Collagenase from the gram-negative bacterium Grimontia hollisae strain 1706B (Ghcol) degrades collagen more efficiently even than clostridial collagenase, the most widely used industrial collagenase. Collagenase (Enzyme Commission number: 3.4.24.3) cleaves the triple-helical region of collagen under physiological conditions, catalyzing the hydrolysis of peptide bonds with glycine residues at the P1 position. It produces the collagenase Ghcol, which consists of 767 amino acid residues with a single catalytic domain containing the zinc-binding motif H492EYVH496. Here, we report the crystal structures of ligand-free and Gly-Pro-hydroxyproline (Hyp)-complexed Ghcol at 2.2 and 2.4 Å resolution, respectively. These structures revealed that the activator and peptidase domains in Ghcol form a saddle-shaped structure with one zinc ion and four calcium ions.

Crystals of Ghcol complexed with Gly-Pro-Hyp were prepared by soaking the crystals of ligand-free Ghcol in a reservoir solution containing Gly-Pro-Hyp. Unexpectedly, Ghcol binds to two peptides at each of three binding sites, which are present in the active site (a) and in the activator subdomains, Act1 (b) and Act2 (c). The sites are separated by a distance of 15 to 27 Å. In the ligand-complexed Ghcol, we found two Gly-Pro-Hyp molecules, each bind at the active site and at two surfaces on the duplicate subdomains of the activator domain facing the active site, and the nucleophilic water is replaced by the carboxyl oxygen of Hyp at the P1 position. All the bound tripeptides exhibited the same conformation as the Pro-Pro-Gly units in collagen. Notably, the Hyp side chains form more hydrogen bonds than those of Pro in all three binding sites. Tyr555 is involved in hydrogen bonding with OE1 atom of Glu520 both in the ligand-free and ligand-bound Ghcols (2.8 Å), and Tyr564 forms a hydrogen bond with O atom of Hyp in the ligand-bound Ghcol. The OH groups of Tyr476 and Tyr480 form water-mediated hydrogen bonds with OXT of Hyp at P3’. Based on crystallographic analysis of clostridial collagenase, it has been shown that the C1 and C2 subdomains, which constitute the active site, undergo contraction at different levels (ColG > ColT > ColH) upon the binding of a peptidic inhibitor. However, as shown in Figure 4, the binding of tripeptides does not significantly change the structure of the Ghcol active site.

>[2x]AVEQCDLSQFQTTSSNQLMAAIRQQGASCVNALFSADTGVQEAAFSSNHMYNVAQYTRTLAQQYAGGGSDELEALYLYLRAGYYAEFYNSNITFLSWVTPAVKGAVDAFVQNAHFYDNGDAHGKVLNEVIITMDSAGLQHAYLDVVTQWLTRWNAQYAEHWYMRNAVNGVFTLLFGGQWNNQYTSLIGEQTALVTALQAFALDRTKVNSPTEFMAANAARELGRLARYTDATIAPKVTEGLTAIFGQYPSYGDGDAIWLGAADTASYYADCSQFNICGFEDALRDAALNQTFICSDTIKIRSQDMSQAQHLAACDKMAYEESFFHTTLETGNQPVADDHNTQLQVNIFNSDTDYGKYAGPIFGIDTNNGGMYLEGNPANVGNIPNFIAYEASYANPDHFVWNLEHEYVHYLDGRFNMYGDFGTPTELVVWWSEGVAEYVSRVNDNPQAIATIQDGSTYTLAQVFDTTYDGFDVDRIYRWGYLAVRFMFERHPDEVQRMLSATRQGRWAEYKAIISGWANQYQSEFAQWTEALAKGDSGAGNGEGTGSGNEGGGESGGNT;>[4x]GPP;>[4x]GPPGPP>GQDMVSPPPPIADEPLTVNTGIYLIECYSLDDKAETFKVNAFLSLSWKDRRLAFDPVRSGVRVKTYEPEAIWIPEIRFVNVENARDADVVDISVSPDGTVQYLERFSARVLSPLDFRRYPFDSQTLHIYLIVRSVDTRNIVLAVDLEKVGKNDDVFLTGWDIESFTAVVKPANFALEDRLESKLDYQLRISRQYFSYIPNIILPMLFILFISWTAFWSTSYEANVTLVVSTLIAHIAFNILVET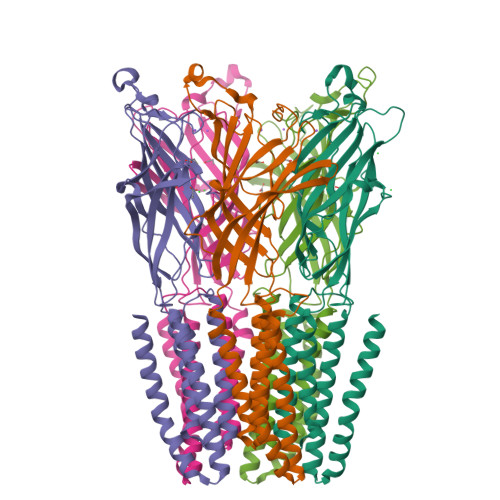NLPKTPYMTYTGAIIFMIYLFYFVAVIEVTVQHYLKVESQPARAASITRASRIAFPVVFLLANIILAFLFFGF[5x]> MSQSNRELVVDFLSYKLSQKGYSWSQMAAVKQALREAGDEFELRYRRAFSDLTSQLHITPGTAYQSFEQVVNELFRDGVNWGRIVAFFSFGGALCVESVDKEMQVLVSRIAAWMATYLNDHLEPWIQENGGWDTFVELYGNNAAAESRKGQER;> XIWIAQELRLIGDLFNAYYARR

In this work we investigate the use of a monosubstituted amino acid in the creation of a hydrocarbon constraint using Bcl-2/BH3 family PPIs as a model. This family of proteins play a pivotal role in the regulation of apoptosis, play a major role in cancer development/progression and represent key targets for anticancer drug-discovery The regulation of apoptosis exploits varying specificity and selectivity of pairwise interactions within the Bcl-2 family interactome. The canonical structural motif involves a BH3 domain from one Bcl-2 family member adopting a helical conformation and binding to a BH3 binding cleft of another partner. In this manuscript we report on the use of a novel α-alkenylglycine derived amino acid to synthesise hydrocarbon constrained BH3-family sequences (BIM and BID). Our biophysical and structural analyses illustrate that whilst the introduction of the constraint increases the population of the bioactive α-helical conformation of the peptide in solution, it does not enhance the inhibitory potency against pro-apoptotic Bcl-xL and Mcl-1 PPIs.

We selected BIM BH3, one of the key BH3 members, as it has a high affinity for all of the anti-apoptotic proteins. Constrained BIM peptides were synthesised by replacing 94Arg and 98Glu with non-natural amino acids. The constrained BIM peptides also showed an increase in helicity as determined by CD, with 57% of BIM-DM and 59% helicity within BIM-MM in comparison to the BIM-WT of 20%. In the case of Bcl-xL/BODIPY-BAK, the constrained BIM variants were less potent, IC50 = 320 nM for BIM-WT, IC50 = 11.9 μM for BIM-MM and IC50 = 4 μM BIM-DM. The constraint itself projects out into solvent and does not contribute to the interaction between the peptide and Bcl-xL. When compared to the structure of Bcl-xL bound to BIM-WT and BIM-DM,43 there are no significant differences in the orientation of hot-spot side chains or registry of the peptide – therefore the reason for the drop in potency is not explained by the static structure of the bound complex. The on rate was also altered in this series of peptides, being 10 times slower with BIM-MM and BIM-DM (2.08 × 104 M s–1 compared to 2.3 × 105 M s–1 for BIM-WT). Crystal structures of Mcl-1/BID-MM and Bcl-xL/BIM-MM revealed that the constrained peptides adopt comparable binding conformations when compared to available structures with wild type sequences and/or peptides constrained with the α,α′-disubstituted alkenyl amino acids. Furthermore our structures confirm that the constraints point away from the BH3 binding cleft and do not introduce steric constraints or new non-covalent interactions with the anti-apoptotic partner.> MRGSHHHHHHLRQCSGKQEWPELVGERGSKAAKIIENENEDVRAIVLPEGSAVPRDLRCDRVWVFVDERGVVVDTPVVM

Recently, attentions have been drawn to another member of the potato inhibitor I family from buckwheat seeds, BWI-1 (Buckwheat Inhibitor 1). Interestingly, BWI-1 has an uncommon binding loop sequence with a Pro at the P2 position and Trp at the P8′ position, suggesting a unique mode of intramolecular interactions between the binding loop and the protein core. Here, we report the crystal structure of rBTI at 1.84 Å resolution and the structure of rBTI-trypsin complex at 2.26 Å resolution. Within the loop, the P1 residue, Arg45, is an ideal substrate of trypsin, which ensures the inhibitor's tight binding to trypsin.

The structure of rBTI is composed of 69 amino acid residues. Its main structural elements comprise a single α-helix (α1, residues 18 to 28), a central parallel β-sheet consisting of two strands (β1, residues 30 to 38; β2, residues 51 to 56), a binding loop (residues 39 to 50) and two irregular structures at the N-terminus (residues 3 to 15) and C-terminus (residues 61 to 69). The Cys4-Cys49 disulfide bond stabilizes the binding loop by connecting it with the N-terminus. The binding loop of rBTI is a convex loop sandwiched between β1 and β2. As in other canonical inhibitors, the binding loop of rBTI forms a hydrogen-bonding network with the protein core. In free rBTI, a water molecule forms hydrogen bonds with Trp53 at the P8′ position, Arg51 at the P6′ position, the α carbonyl oxygen of Pro44 at the P2 position and the α carbonyl oxygen of Asp46 at the P1′ position. This water molecule mediates the interactions between the binding loop and the protein core, stabilizing the structure of the binding loop. However, in the case of rBTI, there is a Pro at the P2 position instead of Thr. Therefore, no hydrogen bond can be formed between the P2 and P8′ residues or between the P2 and P6′ residues, resulting in an extended binding loop distant from the protein core. After superposing LUTI over rBTI, we observed that the binding loop of rBTI was approximately 3.5 Å more distant from the protein core than that of LUTI.Burkholderia pseudomallei is a serious, difficult to treat Gram‐negative pathogen and an increase in the occurrence of drug‐resistant strains has been detected. We have directed efforts to identify and to evaluate potential drug targets relevant to treatment of infection by B. pseudomallei. We have selected and characterised the essential enzyme d‐alanine‐d‐alanine ligase (BpDdl), required for the ATP‐assisted biosynthesis of a peptidoglycan precursor. In a similar manner to that observed previously in other studies, we note a paucity of hits that are worth follow‐up and then in combination with a computational analysis of the active site, we conclude that this ligase represents a difficult target for drug discovery.

A recombinant supply of protein supported high‐resolution crystallographic and biophysical studies with ligands (AMP and AMP+d‐Ala‐d‐Ala), and comparisons with orthologues enzymes suggest a ligand‐induced conformational change occurring that might be relevant to the catalytic cycle.

>MSGIDPKRFGKVAVLLGGDSAEREVSLNSGRLVLQGLRDAGIDAHPFDPAQRPLAALKDEGFVRAFNALHGGYGENGQIQGALDFYGIRYTGSGVLGSALGLDKFRTKLVWQQTGIPTPPFETVMRGDDYAARAQDIVAKLGVPLFVKPASEGSSVAVEKVKSADALPAALEEAAKHDKIVIVEKSIEGGGEYTACIAADLDLPLIRIVPAGEFYDYHAKYIANDTQYLIPCGLDAAKEAEFKRIARRAFDVLGCTDWGRADFMLDAAGNPYFLEVNTAPGMTDHSLPPKAARAVGIGYSELVVKVLSLTLD[2x]> GPLHMGGSPEFPGRLEAADPMSGGLLKALRSDSYVELSQYRD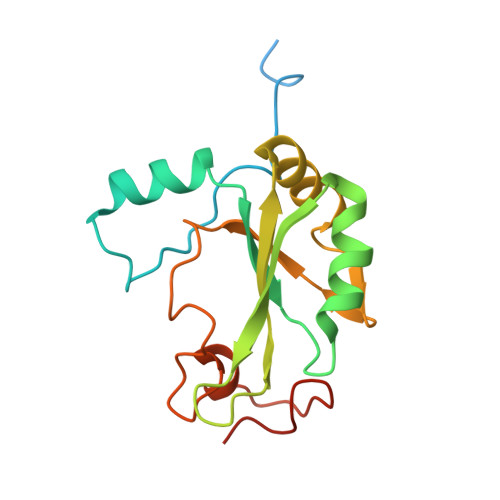QHFRGDNEEQEKLLKKSCTLYVGNLSFYTTEEQIYELFSKSGDIKKIIMGLDKMKKTACGFCFVEYYSRADAENAMRYINGTRLDDRIIRTDWDAGFKEGRQYGRGRSGGQVRDEYRQDYDAGRGGYGKLAQNQ>MHKLLLALLSLSLVGCIDSKEEILEEKNQGLVYCAEANPVSFNPQVTTTGSTIDIIANQLYDRLISIDPVTAEFKSELATDWKISKDGKSVTFTLRKGVKFHTTAYFTPTREFNADDVIFTFSRLFDVYNPYHFVGDANYPYFQSVGIDQLIRKIVRVSDHQVRFELFNAESSFLANMATDFAVVLSKEYAMALKANNQENLFDQYPVGTGPYIYKEYRRDHLVRFYKNADYWKHEVALEQLVYDITPNGTTRIAKILTKECDVTAHPSSAQLSILAQRDDINVERETNLNIGYWAFNTERPPFDNLKVRQALVHAIDIEKIMQAVYYGNGLRARSILPPTSWAFEPQKNMPIFDPQLAKKLLTEAGYEKGFDMSIWAMPVSRIYNPNARKMAELMQSDLRKIGVNVNIVEYEWNTFIQRIGEHRHDSVLLGWAADTPDPDNFFSPLLSCTATFSGKNPANWCNPEFDLLLTKALDTTDLNLRKQYYDAAQSMIIEQLPLYPIAHGMRFQAS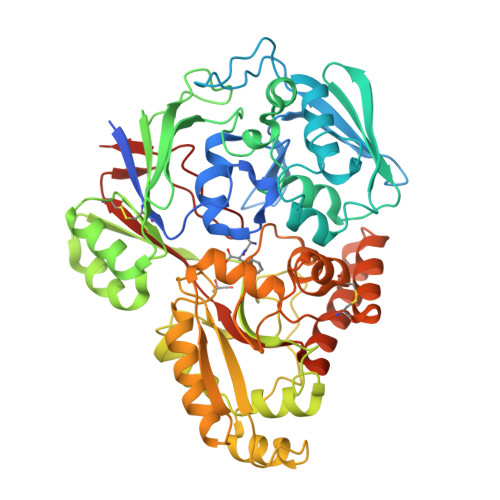SADVEGITLGPFGAISLANARKKHHHHHH[2x]>[3x]SSPADSYNEGVKLQPQEISPPPTANLDRSNDKVYENVTGLVKAVIEMSSKIQPAPPEEYVPMVKEVGLALRTLLATVDETIPLLPASTHREIEMAQKLLNSDLGELINK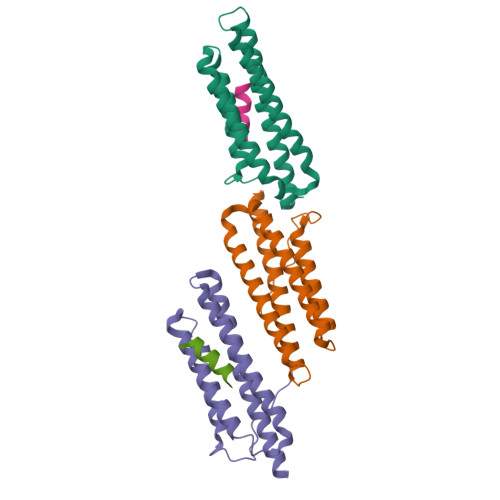MKLAQQYVMTSLQQEYKKQMLTAAHALAVDAKNLLDVIDQARLKMLGQTRPH;>NLSELDRLLLELN[2x]>[11x]MAKRRKIKPMDDEQVLRHLDQLVNDALDFNSSELSKQRSEALKYYFGEPFGNERPGKSGIVSRDVQETVDWIMPSLMKVFTSGGQVVKYEPDTAEDVEQAEQETEYVNYLFMRKNEGFKVMFDWFQDTLMMKTGVVKVYVEEVLKPTFERFSGLSEDMVADILSDPDTSILAQSVDDDGTYTIKIRKDKKKREIKVLCVKPENFLVDRLATCIDDARFLCHREKYTVSDLRLLGVPEDVIEELPYDEYEFSDSQPERLVRDNFDMTGQL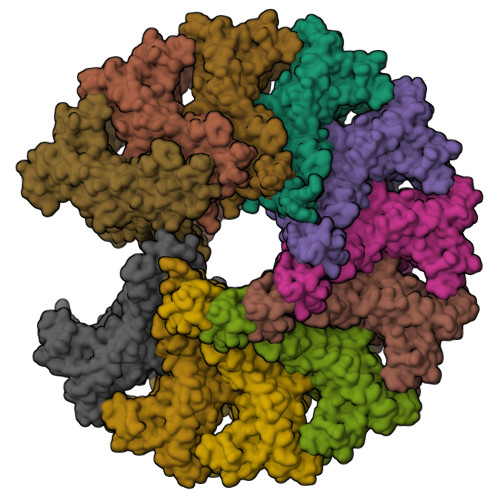QYNSGDDAEANREVWASECYTLLDVDGDGISELRRILYVGDYIISNEPWDCRPFADLNAYRIAHKFHGMSVYDKIRDIQEIRSVLMRNIMDNIYRTNQGRSVVLDGQVNLEDLLTNEAAGIVRVKSMNSITPLETPQLSGEVYGMLDRLEADRGKRTGITDRTRGLDQNTLHSNQAAMSVNQLMTAAEQQIDLIARMFAETGVKRLFQLLHDHAIKYQNQEEVFQLRGKWVAVNPANWRERSDLTVTVGIGNMNKDQQMLHLMRIWEMAQAVVGGGGLGVLVSEQNLYNILKEVTENAGYKDPDRFWTNPNSPEALQAKAIREQKEAQPKPEDIKAQADAQRAQSDALAKQAEAQMKQVEAQIRLAEIELKKQEAVLQQREMALKEAELQLERDRFTWERARNEAEYHLEATQARAAYIGDGKVPETKKPTKAVRR>[2x]GMPQTLKPDTPAGTPAAGAVAFRRQVLPQDALLVRR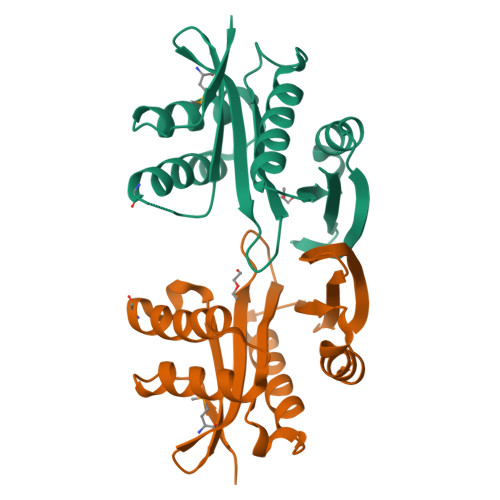VVESTGFFTPEEADVAQELVDEHLMHGAACGYHFVFATEDDDMAGYACYGPTPATEGTYDLYWIAVAPHRQHSGLGRALLAEVVHDVRLTGGRLLFAETSGIRKYAPTRRFYERAGFSAEAVLKAFYRAGDDKIIYRLEVA heptanenitrile | C7 H13 N | 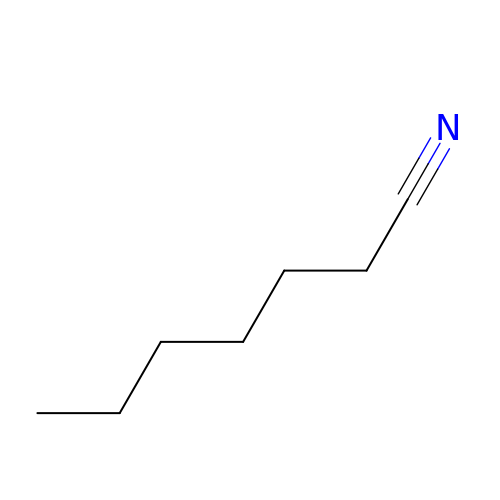SDAXRHHPNYTELL-UHFFFAOYSA-N>[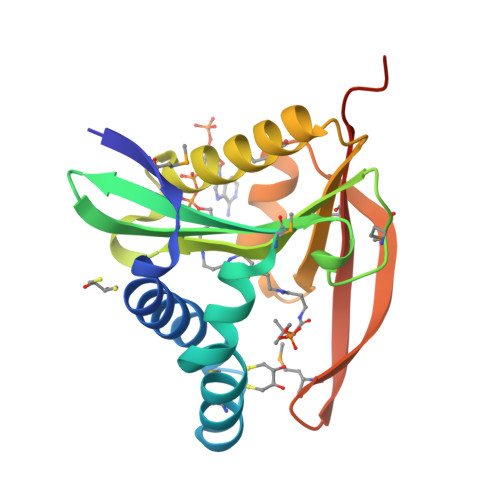2x]MSVKMKKCSREDLQTLQQLSIETFNDTFKEQNSPENMKAYLESAFNTEQLEKELSNMSSQFFFIYFDHEIAGYVKVNIDDAQSEEMGAESLEIERIYIKNSFQKHGLGKHLLNKAIEIALERNKKNIWLGVWEKNENAIAFYKKMGFVQTGAHSFYMGDEEQTDLIMAKTLILEHHHHHH>[4x]DDVDLAEVEKQILATPGVKSFHDLHIWALTSGKASLTVHVVNDTAVNPEMEVLPELKQ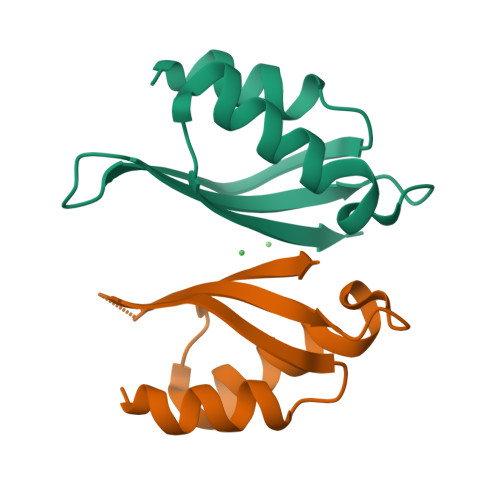MLADKFDITHVTIQFEL> GPGSEENEDSDPLPDNWEMAYTEKGEVYFIDHNTKTTSWLDPRLAKKAKPPEECKENELPYGWEKIDDPIYGTYYVDH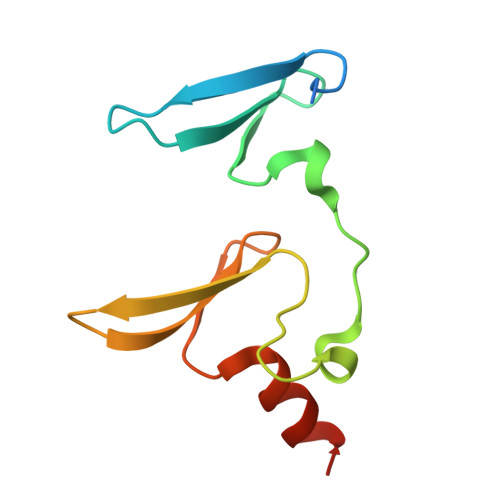INRRTQFENPVLEAKRKLQQHN> MEFSQIPASEQETLVRPKPLLLKLLKSVGAQKDTYTMKEVLFYLGQYIMTKRLYDEKQQHIVYCSNDLLGDL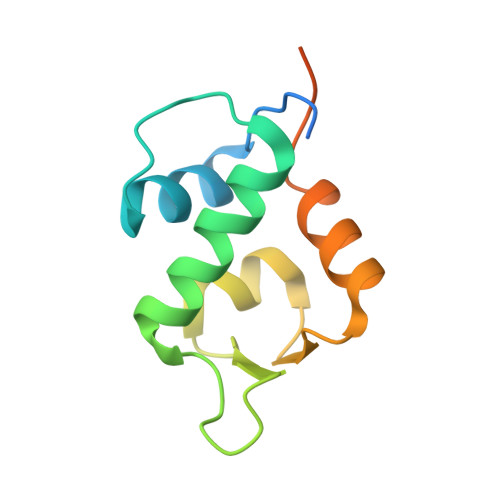FGVPSFSVKEHRKIYTMIYRNLVVVNQQESSDSGTSVSENLE> KIPLTA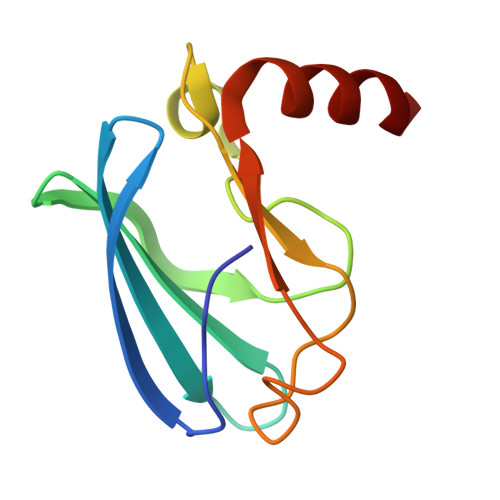VPNQAISFNAGSSYWKIRLYQNMDMMNADISRDGVIVCHGVRCFGGIPLLQYSHQYRPDYGNFVFDRDADWTLFGDGINLFYLDGAEFAEYQALAT> GGHNVAWDYDNNVIRGVNLGGWFVLEPYMTPSLFEPFQNGNDQSGVPVDEYHWTQTLGKEAALRILQKHWSTWITEQDFKQISNLGLNFVRIPIGYWAFQLLDNDPYVQGQVQYLEKALGWARKNNIRVWIDLHGAPGSQNGFDNSGLRDSYNFQNGDNTQVTLNVLNTIFKKYGGNEYSDVVIGIELLNEPLGPVLNMDKLKQFFLDGYNSLRQTGSVTPVIIHDAAQVFGYWNNFLTVAEGQWNVVVDHHHYQVFSGGELSRNINDHISVACNWGWDAKKESHWNVA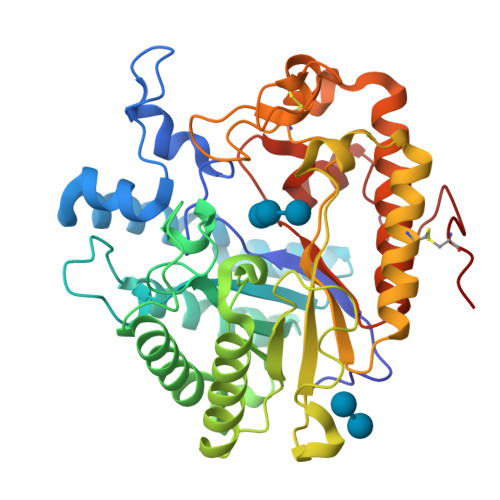GSWSAALTDCAKWLNGVNRGARYEGAYDNAPYIGSCQPLLDISQWSDEHKTDTRRYIEAQLDAFEYTGGWVFWSWKTENAPEWSFQTLTYNGLFPQPVTDRQFPNQCGFH>[3x]GPDEARRQIVSNALISEIAGIVDFVAEEQITVIEQGIEKEITNPLYEQSSGIPYINRTTNKDLNSTMSTNASEFINWGAGTSTRIFFTRKYCISTGTQGNYEFSKDYIPCEEPAILSNSDLKIDRIDFVATDNTVGSAIERVDFILTFDKSNANESFYFSNYVSSLEKAAEQHSISFKDIYVVERNSSGAAGWRLTTISGKPLTFSGLSKNIGSLDKTKNYGLRLSIDPNLGKFLRADGRVGADKLCWNIDNKMSGPCLAADDSGNNLVLTKGKGAKSNEPGLCWDLNTGTSKLCLTQIEGKDNNDKDASLIKLKDDNGNPATMLANILVEEKSMTDSTKKELRTIPNTIYAAFSNSNASDLVITNPGNYIGNVTSEKGRIELNVQDCPVSPD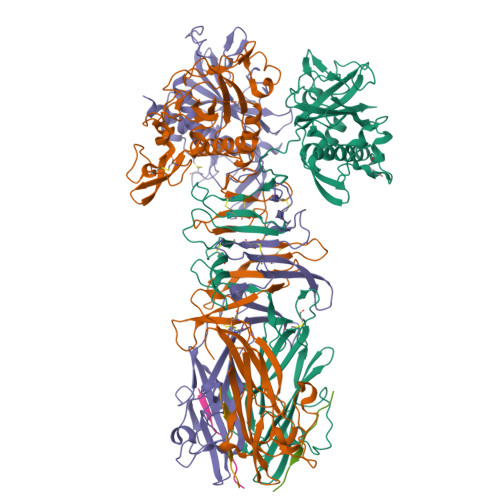GNKLHPRLSASIASIVADTKDSNGKYQADFSSLAGNRNSGGQLGYLSGTAIQVNQSGSKWYITATMGVFDPLTNTTYVYLNPKFLSVNITTWCSTEPQT;>[3x]SPSSSEGGAFTVNMPKTSTVDDIR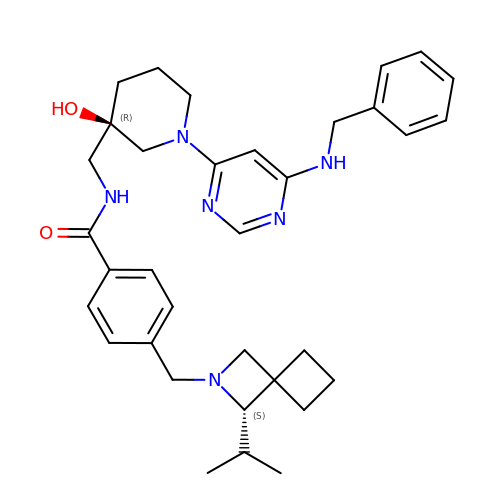N-(((R)-1-(6-(benzylamino)pyrimidin-4-yl)-3-hydroxypiperidin-3-yl)methyl)-4-(((S)-1-isopropyl-2-azaspiro[3.3]heptan-2-yl)methyl)benzamide | C34 H44 N6 O2 | HVTLFMVGWJQMMA-AFPLUKJUSA-N> MTDPVRRDPTEFLRVLRRMSRTTSWQKTMLFASKGRMVGYRLTREHYNTVLFSQSLWGRALEIVRVVRAMQEDKVQPNGATYYYIVNGMGNADHGWNYDFRINRRLEKIQHWRVALEALEACEANGFDSTDTMHNSALITLVIPGFNRWQQA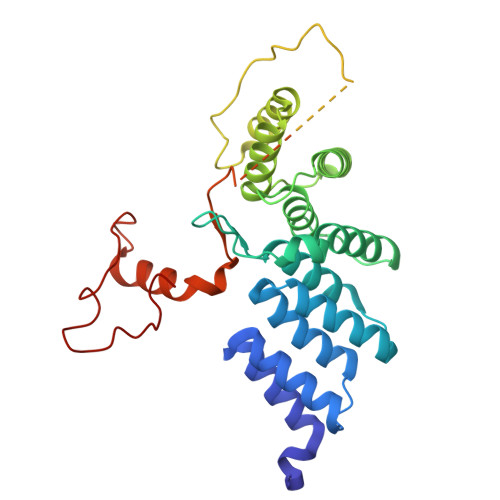SLLLQRMLREDRRMHPTMVKFYHDCLVRNNRPREASSLMRLAAERGVHGYEDKWEADVYKGRPLDSEVMNESEGNGLRRQASSLAFASLMLRGDQRPLPENLQALLEEETTRNIEAERSVPVPFSAGLHATEINSVFRPRVYRQLWYKWQHIANRYRPTAALKRRQLAPRDSPTGIPGFYRI>[2x]MTNGDNLAQIGVVGLAVMGSNLARNFARNGNTVAVYNRSTDKTDKLIADHGSEGNFIPSATVEEFVASLEKPRRAIIMVQAGNATDA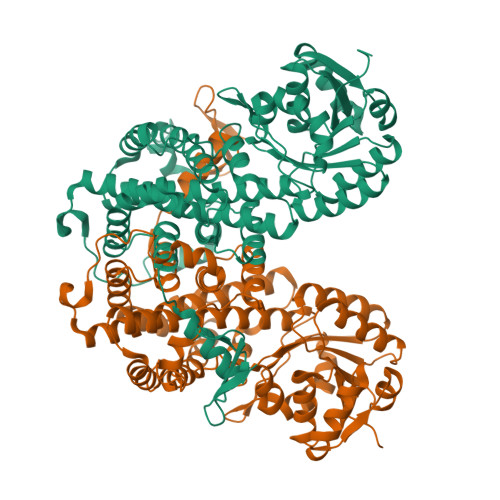VINQLADAMDEGDIIIDGGNALYTDTIRREKEISARGLHFVGAGISGGEEGALNGPSIMPGGPAKSYESLGPLLESIAANVDGTPCVTHIGPDGAGHFVKMVHNGIEYADMQVIGEAYHLLRYAAGMQPAEIAEVFKEWNAGDLDSYLIEITAEVLSQVDAETGKPLIDVIVDAAGQKGTGRWTVKAALDLGIATTGIGEAVFARALSGATSQRAAAQGNLPAGVLTDLEALGVDKAQFVEDVRRALYASKLVAYAQGFDEIKAGSDENNWDVDPRDLATIWRGGCIIRAKFLNRIVEAYDANAELESLLLDPYFKSELGDLIDSWRRVIVTATQLGLPIPVFASSLSYYDSLRAERLPAALIQGQRDFFGAHTYKRIDKDGSFHTEWSGDRSEVEALEHHHHHH> MSNCELTVLKPAEVKLSPRDREGIINPMYDCQPAGAQYAGIGIKDCIPLVHGGQGCTMFVR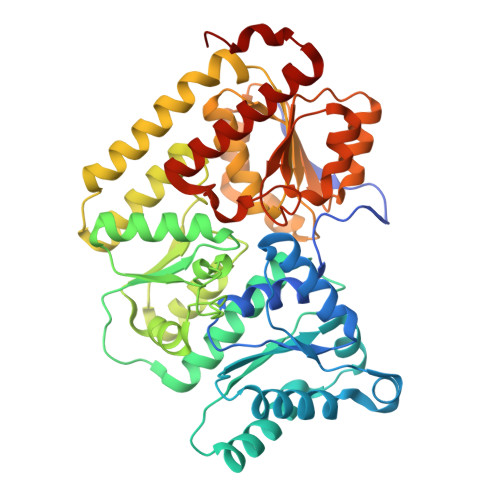LLFAQHFKENFDVASTSLHEESAVFGGAKRVEEGVLVLARRYPNLRVIPIITTCSTEVIGDDIEGSIRVCNRALEAEFPDRKIYLAPVHTPSFKGSHVTGYAECVKSVFKTITDAHGKGQPSGKLNVFPGWVNPGDVVLLKRYFKEMDVEANIYMDTEDFDSPMLPNKSIETHGRTTVEDIADSANALATLSLARYEGNTTGELLQKTFAVPNALVNTPYGIKNTDDMLRKIAEVTGKEIPESLVRERGIALDALADLAHMFFANKKVAIFGHPDLVLGLAQFCMEVELEPVLLLIGDDQGNKYKKDPRIEELKNTAHFDIEIVHNADLWELEKRINAGLQLDLIMGHSKGRYVAIEANIPMVRVGFPTFDRAGLYRKPSIGYQGAMELGEMIANAMFAHMEYTRNKEWILNTW> MKEVNVRESSQEREQRIQQQWQKGNVFQQSVQNREGYPSFVFYEGPPTANGLPHVGHALGRTIKDVVARYKTMTGHQVIRKAGWDTHGLPVELGVEKQLGISGKHDIEKYGVEAFINKCKESVFVYEKQQRTFTEQLGYWVDMEDPYITLENSYIESVWNVLGTIHDKGLLYKGHRVSPYCPSCQTSLSSHEVAQGYKDVKDLTVTVKFKVKNRDNEYFLGWTTTPWTLPSNVALAVHEEMSYVRAEQGDSVYIVAEALADKVLKGEYSVLSHHKGNELKGMSYEPPFNFVKVEKGHEVVTADYVTDQSGTGVVHLAPAYGEDDYRVVKENGFSFVNVVDEKGQYTSEVPPFQGRFVKDCDVDIVRYLANQDVLYHKEKHEHSYPFCWRCDSPLLYYANESWFIQTTALKEQFLKNNESVKWYPDHIKHGRFGKFLENMVDWNISRKRYWGTPLNVWECEGCQHQVAPKSIKELQKHASHYVDDSIELHKPYVDDVQLTCPVCSGEMKRTPEVIDVWFDSGSMPFAQYHYPFENSELFQKQFPADVIAEGIDQTRGWFYSLMAVSTLFTGKAPYKRVLSLGHVLDENGQKMSKSKGNALDPVDLIHTFGADALRWALLADSAPWNPKKFSERVVQEAKSKVIDTLVNVYGFYVLYAKLDGYDPEQTYELKKTKLDEWILSRLHSTVKRATVHLEDYGFTSAAREIAVFIEELSNWYVRRSRDRFWSEGMDGEKAAAYDTLHEVLVTLSQLLAPFTPFVADDVHENLTGKSVHLADYPACDQTKVNEKLEKEMAAVLQVVELGRSIRNTHSLKVKQPLQSLSLVVTEEDVEWKAYRDVIKDELNVKNFNVEQDDDKLVSYVLKLDFKQAGPKFGKQVNEVNQALKNLSEEKGKEFVEQGKLSVTLASGENLTLETEDVLVEKVPKEGFAVASNGMYTAVLDTALTEELVQEGVAREVIRAVQDYRKKLDLPVNSRINLELSGDEEVQKAVAKFETLLQENLLLHSLSVKETIKNGETVKVGTKQVVLRVLNQS

Mupirocin, a clinically used natural antibiotic, inhibits isoleucyl-tRNA synthetase (IleRS), an enzyme that links isoleucine to its tRNAIle for protein synthesis. Two IleRSs, mupirocin-sensitive IleRS1 and resistant IleRS2, coexist in bacteria. Specifically, type 1 proteins (IleRS1) are strongly inhibited by mupirocin (Ki in low nanomolar range), while IleRS2, which are homologous to IleRSs from the eukaryote cytosol, exhibit resistance to mupirocin concentrations that are about three orders of magnitude higher. AARSs catalyze the formation of AA-tRNA in two steps within the same active site. The amino acid is first activated by ATP to form an aminoacyl-adenylate (AA-AMP) intermediate, followed by the transfer of the aminoacyl moiety to the tRNA.

The displacement (shift) of the HIGH motif in IleRS2 is of utmost importance for the accommodation of the non-canonical A/GXHH motif and emergence of hyper-resistance. Hence, to explore it further, we extensively analyzed the residues in the immediate vicinity of the HXGH motif using mutagenesis combined with biochemical and structural characterization (exemplified for the W130Q-PmIleRS2 mutant in Supplementary Fig. 8 and Supplementary Table 2).> AHYNTEILKSIDNEWRKTQCMPREVAIDVGK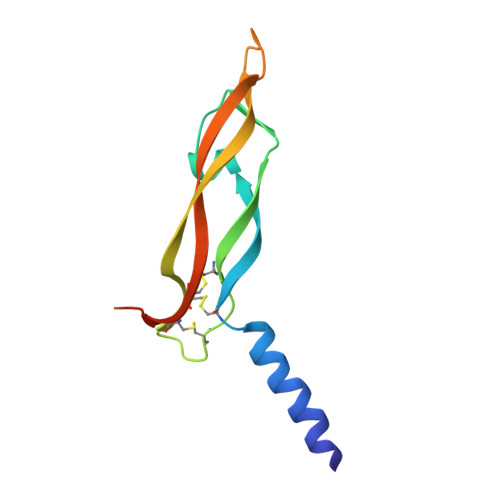EFGVATNTFFKPPCVSVYRCGGCCNSEGLQCMNTSTSYLSKTLFEITVPLSQGPKPVTISFANHTSCRCMSKLHHHHHH> DGVSILQTASSGLTSLTNSLQRIRQLAVQASNGPLSASDASALQQEVAQ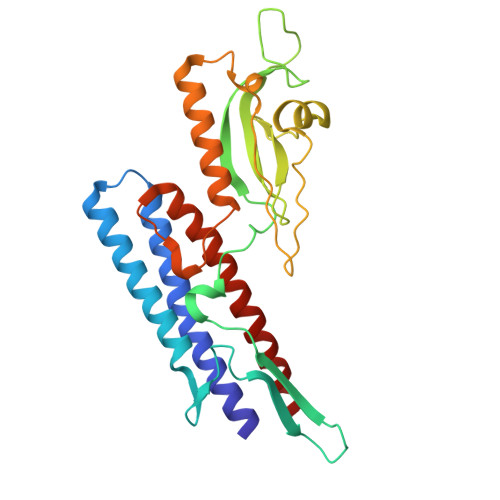QISEVNRIASQTNYNGKNILDGSAGTLSFQVGANVGQTVSVDLTQSMSAAKIGGGMVQTGQTLGTIKVAIDSSGAAWSSGSTGQETTQINVVSDGKGGFTFTDQNNQALSSTAVTAVFGSSTAGTGTAASPSFQTLALSTSATSALSATDQANATAMVAQINAVNKPQTVSNLDISTQTGAYQAMVSIDNALATVNNLQATLGAAQNRF>MGPLPRTVELFYDVLSPYSWLGFEILCRYQNIWNINLQLRPSLITGIMKDSGNKPPGLLPRKGLYMANDLKLLRHHLQIPIHFPKDFLSVMLEKGSLSAMRFLTAVNLEHPEMLEKASRELWMRVWSRNEDITEPQSILAAAEKAGMSAEQAQGLLEKIATPKVKNQLKETTEAACRYGAFGLPITVAHVDGQTHMLFGSDRMELLAHLLGEKWMGPI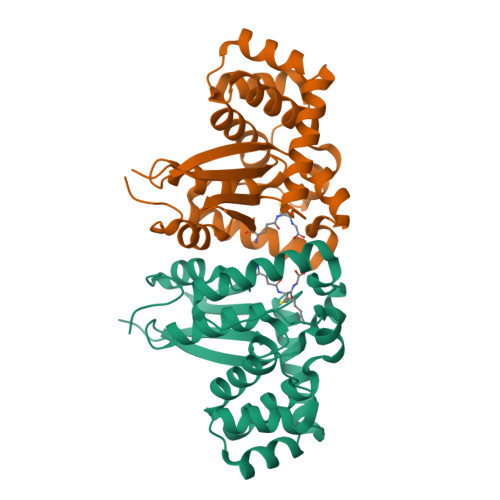PPAVNARLLEHHHHHH[6x]> MTMKQLTNSMDMMRQACAPKFKVEEAELHGLRKSIFPANPDKELKCY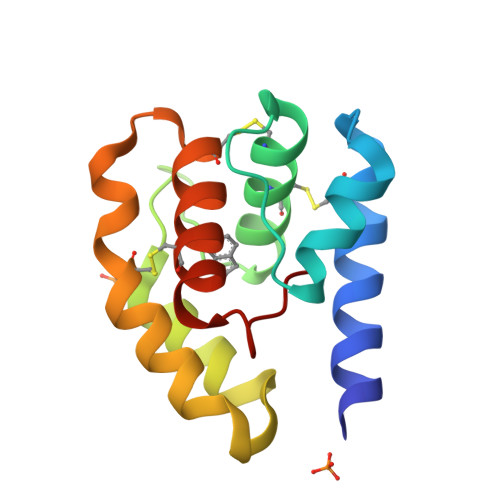AMCIAQMAGTMTKKGEISFSKTMAQIEAMLPPEMKTMAKEALTHCKDTQTSYKDPCDKAYFSAKCAADFTPDTFMFP>[6x]AARAPSVSAKPGPALWPLPLSVKMTPNLLHLAPENFYISHSPNSTAGPSCTLLEEAFRRYHGYIFGFYKWHHEPAEFQAKTQVQQLLVSITLQSECDAFPNISSDESYTLLVKEPVAVLKANRVWGALRGLETFSQLVYQDSYGTFTINESTIIDSPRFSHRGILIDTSRHYLPVKIILKTLDAMAFNKFNVLHWHIVDDQSFPYQSITFPELSNKGSYSLSHVYTPNDVRMVIEYARLRGIRVLPEFDTPGHTLS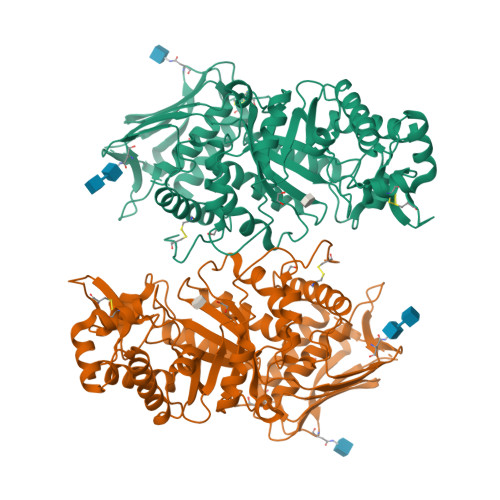WGKGQKDLLTPCYSRQNKLDSFGPINPTLNTTYSFLTTFFKEISEVFPDQFIHLGGDEVEFKCWESNPKIQDFMRQKGFGTDFKKLESFYIQKVLDIIATINKGSIVWQEVFDDKAKLAPGTIVEVWKDSAYPEELSRVTASGFPVILSAPWYLDLISYGQDWRKYYKVEPLDFGGTQKQKQLFIGGEACLWGEYVDATNLTPRLWPRASAVGERLWSSKDVRDMDDAYDRLTRHRCRMVERGIAAQPLYAGYCNHENM> GSSG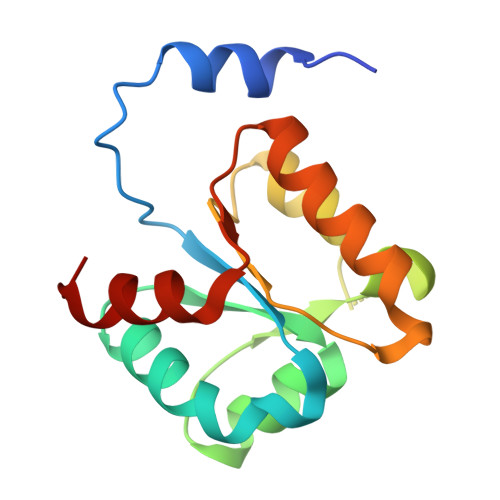SSGHTAFLKAMLSTGFKIPQKGILIGIQQSFRPRFLGVAEQLHNEGFKLFATEATSDWLNANNVPATPVAWPSQEGQNPSLSSIRKLIRDGSIDLVINLPNNNTKFVHDNYVIRRTAVDSGIPLLTNFQVTKLFAEAVQ>[3x]MALVKATFVKDVDGQPWRFSSVAKMKAFNYSCYLGSSVFLESWHEGAGLGSGLFKVSKGTTEVGDDGSVIVAADGTRLIRVFDGPIFADMWGALPSSTYNSLPAIKSAYLYASSKLQQLFLGGGSYKVTGSSGIDIDPSLAGISALSRARVDTTEFTGDYLFTITSSYSYTPAPYYNNLSVALEGLYVFGNKTEGRSGLLTGRRTTDGVKSYNGQTEIRNCTFDKFDYNIRMGHNSWRIVFYKVNSLNALNANGILYVPSGLDDSGEILTFYHCQFFDGAGSNIRISCSSFAMTFVSCSFLNITFTIDAGSSVSVTALGCNFENP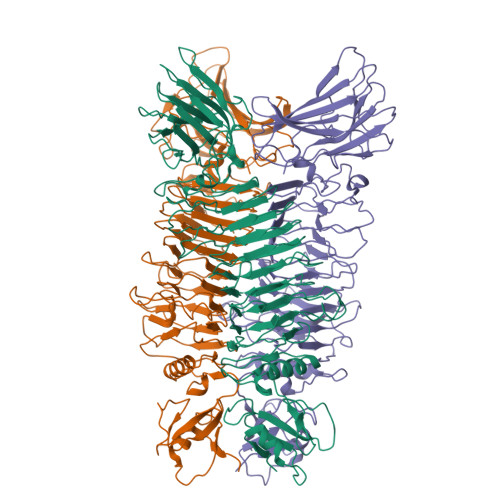GSQSTRRYIEITAGHTNIFNVVGGSIVTNANAGQTQALIHVSANNQINLSNLTIPYGAHYQQEADSGYHAFCSGQGYVSTSNCSLQLLNGAGCCPIHPSLSVFTNWNLSYANLNAWTVDKGSAPTSVAEYLSAQGPKGEGVLHVAPTTQGVNISQVATVSKQAGSMSMSVMVNIISASSNAGQISLAYLDAFDNNLGGVSANLGTTTGWKVIGKNTLRGRLPVGTAKVRLNIQTVAGADVQYTNILCNII> HHHHHHEVLLRSTETGQYLRINPDGTVDGTRDRSDPGIQYQISPEGNGEVLLRST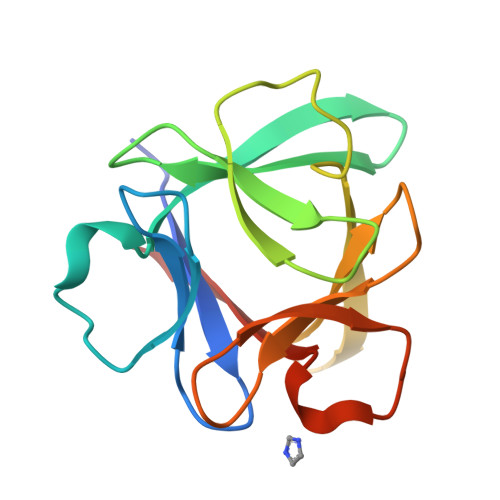ETGQYLRINPDGTVDGTRDRSDPGIQYQISPEGNGEVLLRSTETGQYLRINPDGTVDGTRDRSDPGIQYQISPEGNG> SGKNPVESVSVEFEAKSARDGAWYDVAAFLSHRLFESGDPEVRVRFSGFGAEEDEWINVRKCVRQRSLPCEATECVAVLPGDLILCFQEGKDQALYYDAHVLDAQRRRHDVRGCRCRFLVRYDHDSSEEIVPLR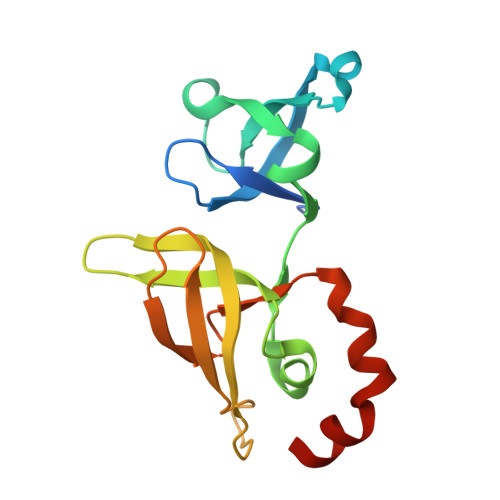KVCRRPETDYRLQILHAARAAATN> SNAMEVTVPATLNVLNGSDARLPCTFNSAYTVNHKQFSLNWTYQECNNCSEEMFLQFRMKIINLKLERFQDRVEFSGNPSKYDVSVMLRNVQPEDEGIY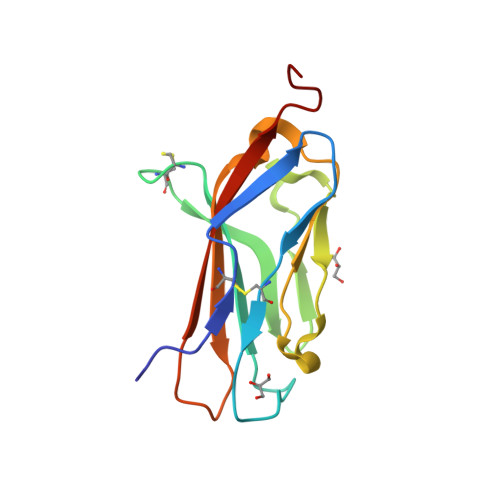NCYIMNPPDRHHGHGKIHLQVLMEEPPE>[2x]GMTQLDTWLANTKPLIPVIVIDDLVHAIPMAKALVAGGVHLLEVTLRTEAGLAAISAIKKAVPEA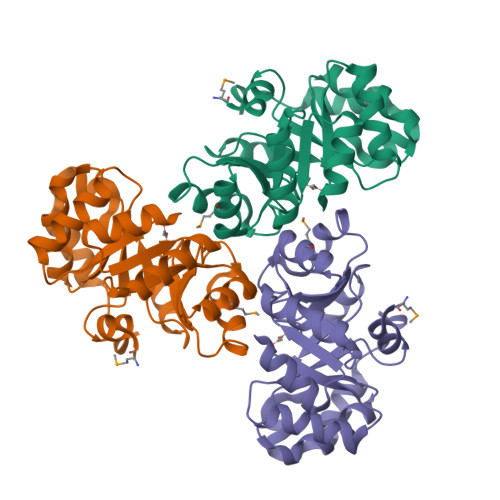IVGAGTVCTADDFQKAIDAGAQFIVSPGLTPELIEKAKQVKLDGQWQGVFLPGVATASEVMIAAQAGITQLKCFPASAIGGAKLLKAWSGPFPDIQFCPTGGISKDNYKEYLGLPNVICAGGSWLTESKLLIEGDWNEVTRRASEIVKLSDI> GPVEDAITAAIGRVADTVGTGPTNSEAIPALTAAETGHTSQVVPSDTMQTRHVKNYHSRSESTIENFLCRSACVYFTEYENSGAKRYAEWVITPRQAAQLRRK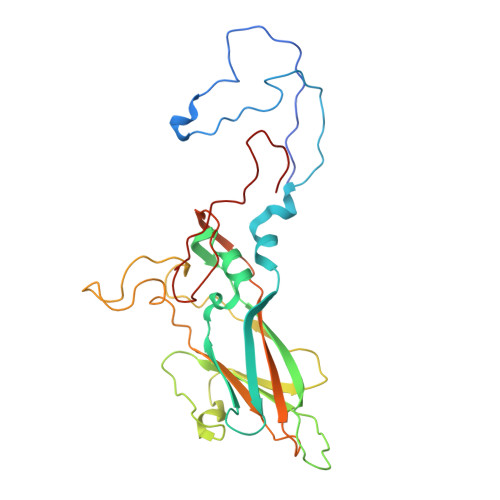LEFFTYVRFDLELTFVITSTQQPSTTQNQDAQILTHQIMYVPPGGPVPDKVDSYVWQTSTNPSVFWTEGNAPPRMSVPFLSIGNAYSNFYDGWSEFSRNGVYGINTLNNMGTLYARHVNAGSTGPIKSTIRIYFKPKHVKAWIPRPPRLCQYEKAKNVNFQPSGVTTTRQSITTMTNT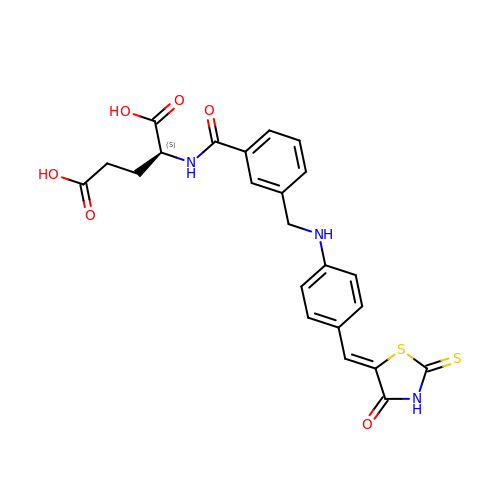N-({3-[({4-[(Z)-(4-oxo-2-thioxo-1,3-thiazolidin-5-ylidene)methyl]phenyl}amino)methyl]phenyl}carbonyl)-L-glutamic acid | C23 H21 N3 O6 S2 | ISIOCNFLEMFKTN-PBXDPIQXSA-N>GSHMDGTEKWRFKTGKAIEASPVIGEDGTIYVGS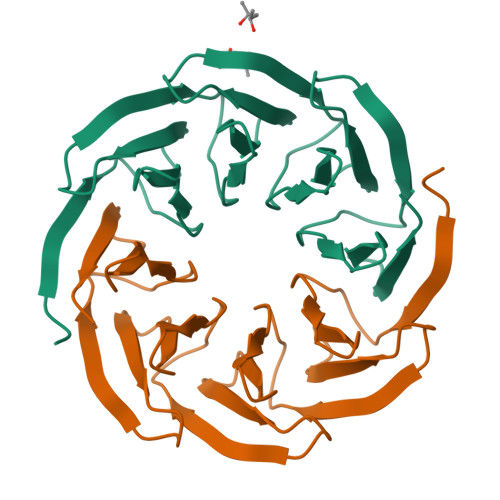NDGHLYAINPDGTEKWRFKTGKAIEASPVIGEDGTIYVGSNDGHLYAINPDGTEKWRFKTGKAIEASPVIGEDGTIYVGSNDGHLYAINPDGTEKWRFKTGKAIEASPVIGEDGTIYVGSNDGHLYAINP[2x]> MLLVKAVKVLVMGGCMLPIAFGALGTGVLFAGFNVALSRNPEETESLFNNTLM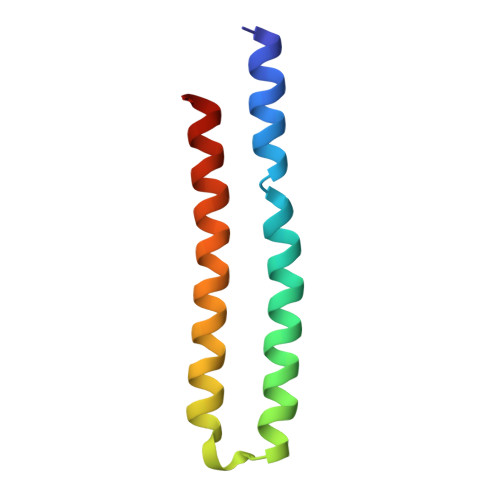GFALIETFIFMSIGLGFFVLFAA> ALITQQDLAPQQRAAPQQKR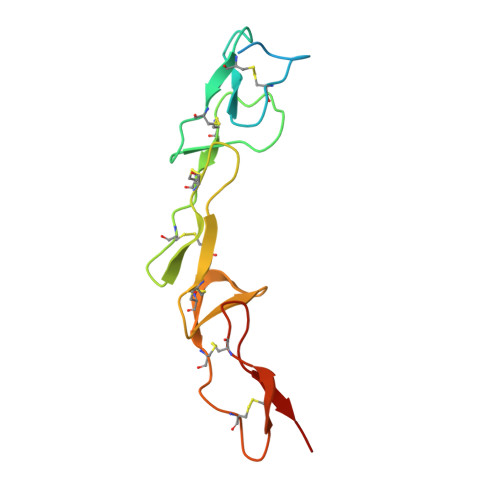SSPSEGLCPPGHHISEDGRDCISCKYGQDYSTHWNDLLFCLRCTRCDSGEVELSPCTTTRNTVCQCEEGTFREEDSPEMCRKCRTGCPRGMVKVGDCTPWSDIECVHKES[[[(2~{R},3~{S},4~{R},5~{R})-5-(6-aminopurin-9-yl)-3-[[(2~{R},3~{S},4~{R},5~{R})-5-(6-azanyl-4,5-dihydropurin-9-yl)-3,4-bis(oxidanyl)oxolan-2-yl]methoxy-oxidanyl-phosphoryl]oxy-4-oxidanyl-oxolan-2-yl]methoxy-oxidanyl-phosphoryl]oxy-sulfanyl-phosphoryl] 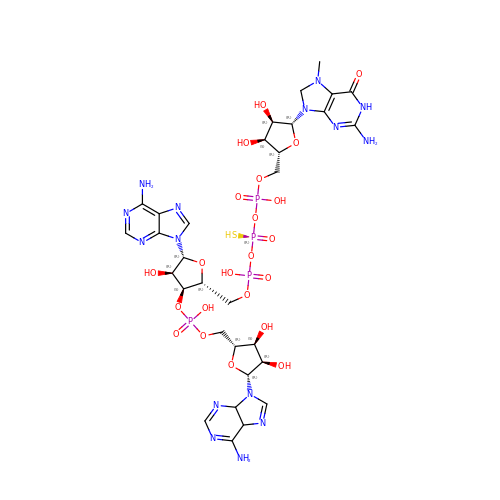[(2~{R},3~{S},4~{R},5~{R})-5-(2-azanyl-7-methyl-6-oxidanylidene-1~{H}-purin-9-yl)-3,4-bis(oxidanyl)oxolan-2-yl]methyl hydrogen phosphate | C31 H45 N15 O22 P4 S | COVMLUYPZIGUSP-PEDZGMCBSA-N> MGDSILSQA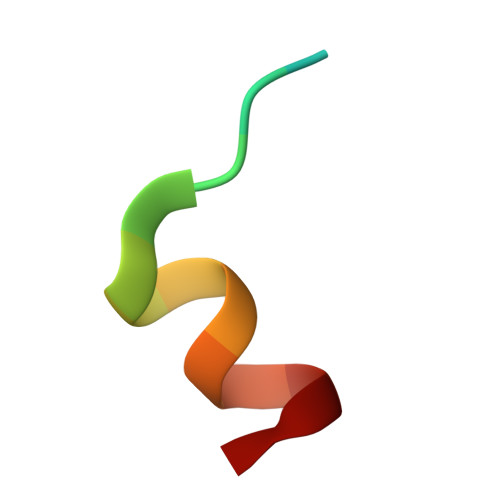EIDALLN> MTWKLASRALQKATVENLESYQPLMEMVNQVTESPGKDDPYPYVVIGDQSSTPFETKSSFGENITMDFHVWGGTTRAEAQDISSRVLEALTY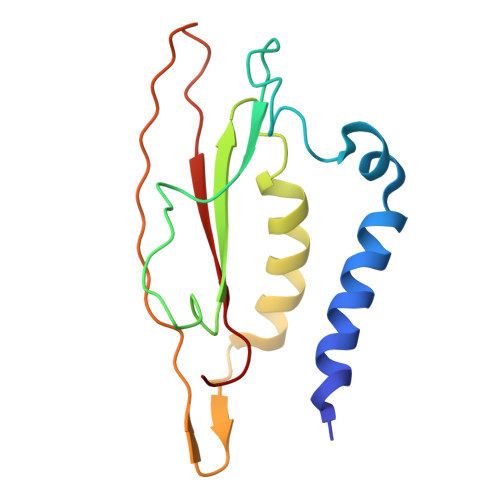KPLMFEGFTFVAKKLVLAQVITDTDGVTKHGIIKVRFTINNN>[2x]MGSSHHHHHHSSGLVPRGSMRIGQYQLRNRLIAAPMAGITDRPFRTLCYEMGAGLTVSEMMSSNPQVWESDKSRL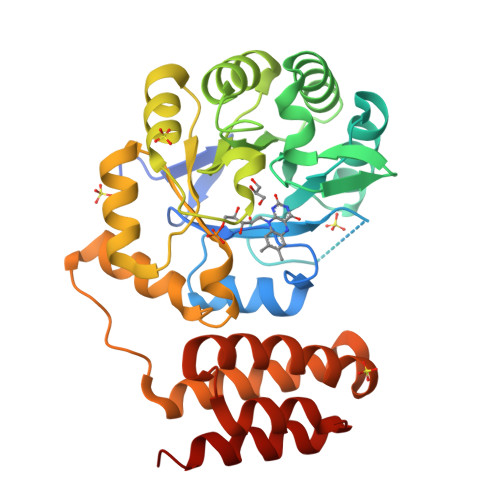RMVHIDEPGIRTVQIAGSDPKEMADAARINVESGAQIIDINMGCPAKKVNRKLAGSALLQYPDVVKSILTEVVNAVDVPVTLKIRTGWAPEHRNCEEIAQLAEDCGIQALTIHGRTRACLFNGEAEYDSIRAVKQKVSIPVIANGDITDPLKARAVLDYTGADALMIGRAAQGRPWIFREIQHYLDTGELLPPLPLAEVKRLLCAHVRELHDFYGPAKGYRIARKHVSWYLQEHAPNDQFRRTFNAIEDASEQLEALEAYFENFA> GSHMASMGVTVQDICFAFLQNYYERMRTDPSKLAYFYASTAELTHTNYQSKSTNEKDDVLPTVKVTGRENINKFFSRNDAKVRSLKLKLDTIDFQYTGHLHKSILIMATG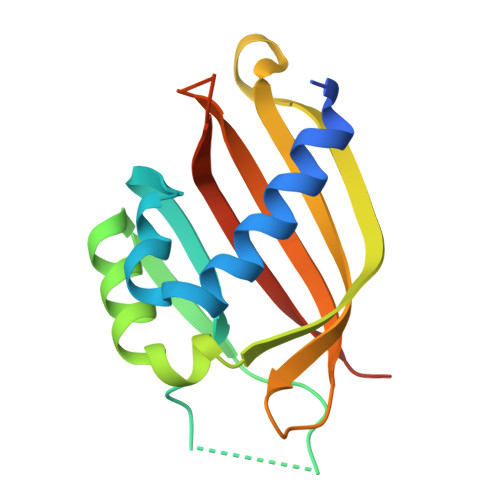EMFWTGTPVYKFCQTFILLPSSNGSTFDITNDIIRFISNSFKLE3-[1-(3-AMINOPROPYL)-1H-INDOL-3-YL]-4-(1H-INDOL-3-YL)-1H-PYRROLE-2,5-DIONE 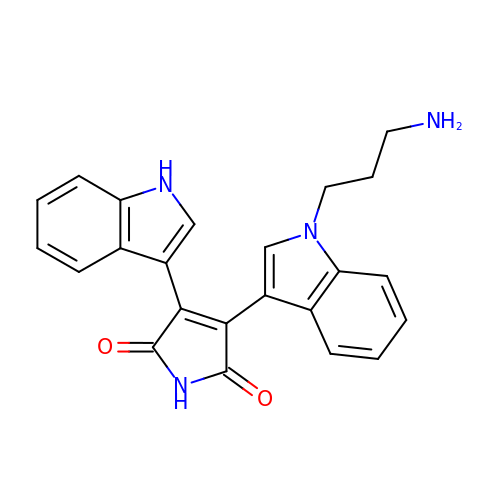| C23 H20 N4 O2 | APYXQTXFRIDSGE-UHFFFAOYSA-N> MGIHLFWDSRVPVGLSRPVSEELSAVLEMPVSRIDDGIFPLEGFDPVRNQYDAVKVLLKLDMFRRRMPQIFKPADMDLE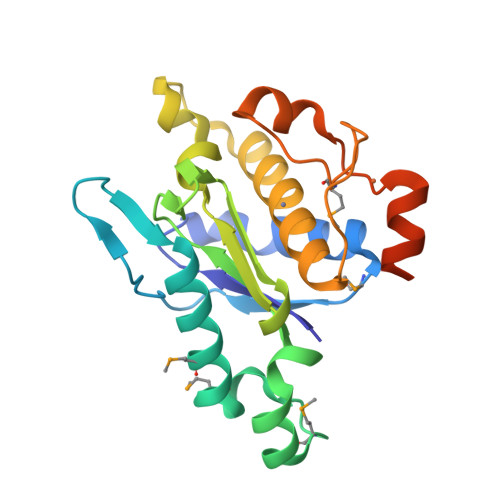FYNKFNHLHEKILLVTPGDLYEPLADFVFGLAYPKLGVAIVSPHRLQNEFYGKYADDSALIDRIVKEGAHEIGHLFGLGHCDNPGCIMYCPRNLDELDRKRKYFCGKCRVQLNGDTLEDDLFSLEHHHHHH Since most proteins are diamagnetic, spin labels such as MTSSL are routinely attached to the surface of proteins via site-directed spin labelling techniques. Thus, the problem arises, that on the one hand, the PELDOR experiment delivers an accurate distance between the two spin centres, but on the other hand, the exact position of the distance vector with respect to the protein is unknown. We present here the high-resolution (1.5 Å) structure of azurin from Pseudomonas aeruginosa PAO1 spin labelled with MTSSL at position T21. Whereas one of the conformations fits to calculated rotamer libraries the second conformation does not, illustrating how the environment of the label can force it to adopt a conformation which is less favourable for the free label.

The asymmetric unit of spin labelled azurin T21R1 contains four independent monomers of azurin (I-IV) that are related by a two-fold NCS axis. Due to the crystal-packing environment in the triclinic crystals, the label is observed in two different but fully ordered states. Following initial refinement with omitted R1 side chain, models of the label could be unambiguously placed into the electron density in all four monomers, resulting in two distinct conformations of the label. In monomers I and III, the label is involved in vdW interactions with residues T126 and K128 of the same monomer and vdW interactions with residues A119 and L120 of a neighboring azurin monomer. Henceforth, the R1 conformation found in monomers I and III will be referred to as R1-I/III. In monomers II and IV, the R1 side chain lies at the heart of a crystal contact and is involved in numerous van-der-Waals (vdW) interactions and a hydrogen bond between the nitroxide oxygen and an ordered water molecule. For this R1 conformation (from here on referred to as R1-II/IV) PISA calculates a solvent accessible surface area of 260 Å2, 171 Å2 of which are buried. In monomers II and IV, the crystal-packing environment precludes the R1-I/III conformation due to steric constraints. Interestingly, the nearby K128 side chain rotates from the position found in monomers I and III by 180° to accommodate the R1-II/IV conformation. Comparison with the rotamer library reveals that χ2, χ4 and to a lesser extend χ5 of R1-II/IV adjust to values that are less favorable for the free label.

>[4x]GAMAECSVDIQGNDQMQFNTNAICVDKSCKQFTVNLSHPGNLPKNVMGHNWVLSTAADMQGVVTDGMASGLDKDYLKPDDSRVIAHTKLIGSGEKDSVTFDVSKLKEGEQYMFFCTFPGHSALMKGTLTLK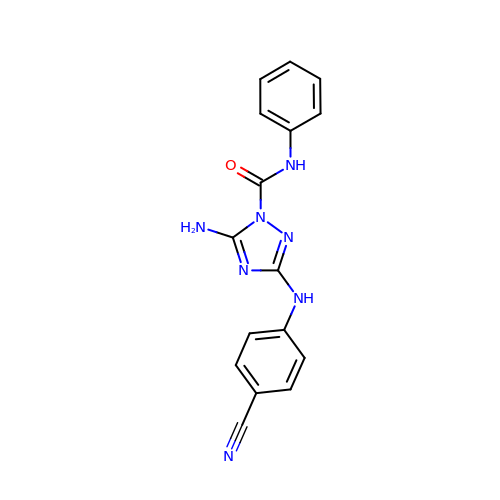5-amino-3-[(4-cyanophenyl)amino]-N-phenyl-1H-1,2,4-triazole-1-carboxamide | C16 H13 N7 O | CYMJSSGSRPDYFG-UHFFFAOYSA-N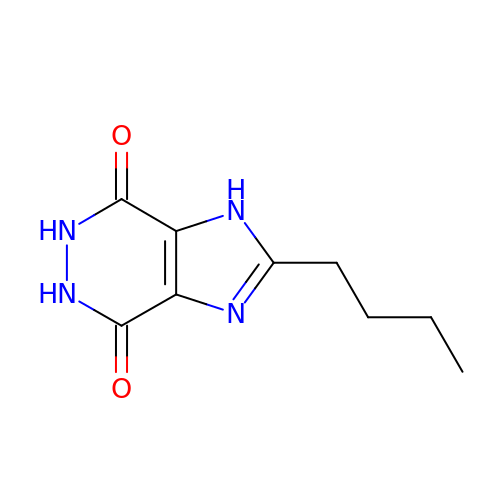2-BUTYL-5,6-DIHYDRO-1H-IMIDAZO[4,5-D]PYRIDAZINE-4,7-DIONE | C9 H12 N4 O2 | DQHJYYALMHIEAH-UHFFFAOYSA-N>[8x]MAPTWFYNTTNSEKLRELQHVLGGSAKLGYLTAKVTEILDVDLETVIRAKAIAAYRAVRVPVIVEHGALCIDALNGLPGALVKPFWESLDT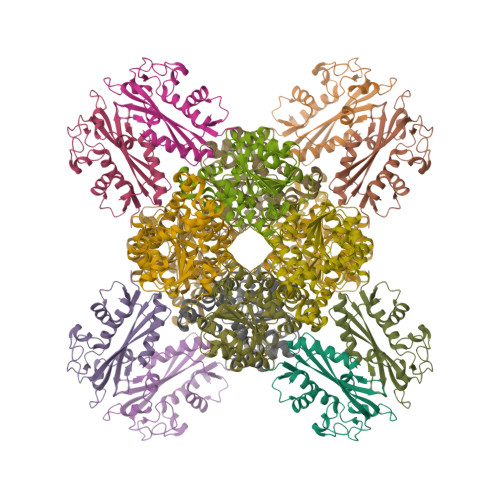RLCEVIPAGQRTARARGALCYCDGRERHVLIEETEGEIAPSARGTGGFHWDPIFIPKGQTRTFAEMSLDEKLSFSPLGRLHTRLRTELGL;>[8x]MTTLTLSEAAPLLKKEFREGRLIPFLGAGFSKPLKLPDGSQLIASLAKTLGFEPELFDMHGRFEQLAEFFAISAPNRLQRLVYEMSLSFDSAEAEALREKSPMHRALAALDWRTIYTTNYDKHVEGALRDAGKQAAVLASFADFQGPRARDVCEVIKFHGTLDQPDTIVLTESSYFQRMALDAPPDQRLRADLLANSFLFIGYSFSDTNIRYIWYRMNQLREQSQLGVKHSQARRCFFATHGAGLVQPDILQQWNIDVIQLDPTDKSASVARLLESIA>[2x]MMVAWWSLFLYGLQVAAPALAATPADWRSQSIYFLLTDRFARTDGSTTATCNTADQKYCGGTWQGIIDKLDYIQGMGFTAIWITPVTAQLPQ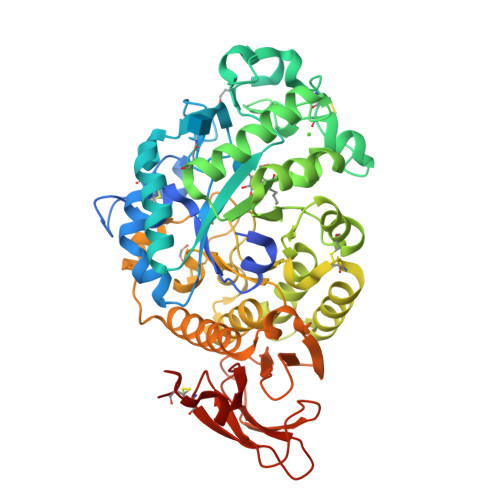TTAYGDAYHGYWQQDIYSLNENYGTADDLKALSSALHERGMYLMVDVVANHMGYDGAGSSVDYSVFKPFSSQDYFHPFCFIQNYEDQTQVEDCWLGDNTVSLPDLDTTKDVVKNEWYDWVGSLVSNYSIDGLRIDTVKHVQKDFWPGYNKAAGVYCIGEVLDGDPAYTCPYQNVMDGVLNYPIYYPLLNAFKSTSGSMDDLYNMINTVKSDCPDSTLLGTFVENHDNPRFASYTNDIALAKNVAAFIILNDGIPIIYAGQEQHYAGGNDPANREATWLSGYPTDSELYKLIASANAIRNYAISKDTGFVTYKNWPIYKDDTTIAMRKGTDGSQIVTILSNKGASGDSYTLSLSGAGYTAGQQLTEVIGCTTVTVGSDGNVPVPMAGGLPRVLYPTEKLAGSKICSSS> MDETGKELVLALYDYQEK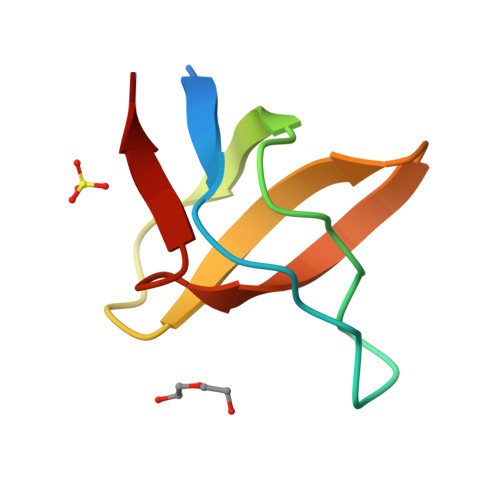SPREVTMKKGDILTLLNSTNKDWWKVEGNGRQGFVPAAYVKKLD> MRGSHHHHHHGSSYQIAVLAGDGIGPEVMAEARKVLKAVEARFGLNIEYTEYDVGGIAIDNHGCPLPEATLKGCEAADAVLFGSVGGPKWEHLPPNDQPERGALLPLRGHFELFCNMRPAKLHPGLEHMSPLRSDISEKGFDILCVRELTGGIYFGKPKGRQGEGENEEAFDTMRYSRKEIRRIAKIAFESAQGRRKKVTSVDKANVLACSV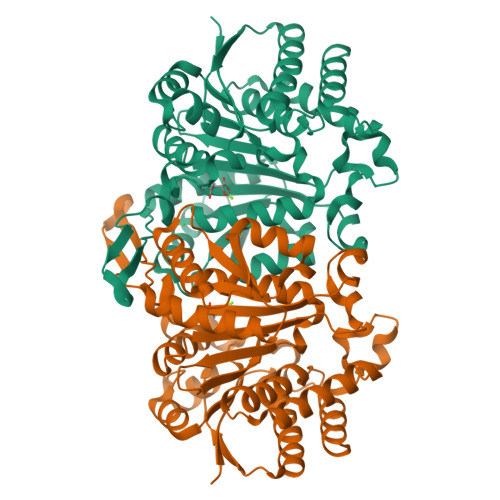LWREVVEEVAKDYPDVELEHIYIDNATMQLLRRPNEFDVMLCSNLFGDIVSDEIAMLTGSMGLLASISMNSQGFGMYEPAGGSAPDIAGQGIANPVAQILSAALLLRHSLKLEDAALAIEAAVSKALNSGYLTGELLSSDQRHKAKTTVQMGDFIADAVKAGV> GETGQVIKSAVRSTVENTVQSTHSITTEATPALQAAETGATSNASDESMIETRNVVNTHGVAETSLEAFYGRAGLVAMFSTDGGIYRWYINFGEYVQLRAKLELLTYARFDMEFTIVAQVVNAQSKVQDFNVDYQVMFVPPGASVPENQDSYQWQSSCNPSVISNTGLPPARVSVPFMSSANAYSFSYDGYTQFGDTSGSSYGIVPSNYLGMLVVRTCEDLDGTRLRVRVYAKPKHVKGWIPRSPRMTPYKSRYTGVYTDTTKFCANRARITTAG;> SAEACGYSDRVAQLTLGNSTITTQEAANIVVGYGRWPTSLRDTDATAVDKPTQPGVSAERFYTLPSVQWTNSFKGHYWKLPDALSELGLFGQNLQFHYLYRGGWVIHVQCNATKFHQGTLLVVATPEHKIQSAESPAFARTNPGEQGAAYQFPFTFEDGTALGNALIYPHQWVNLRTNNSATLVLPYVNALPMDSGIRHNNWTLSVIPIVPLEYAAGATTYVPITVTIAPMCTEYNGLRAAVTQ;> GIPTLYTPGSGQFLTTDDFQTPCMLPKFQPTPVIDIPGEVKNFLEVVQVESLVEINNVESAEGVARYRIPLNVQDAMDGQIMALRVDPGIDGPMQSTLLGVFTRYYAQWSGSLDFTFMFCGTFMTTGKVIIAYTPPGGDQPTNRRQAMLGTHVVWDFGLQSSITLVVPWISSGHFRGTTLENTIYKYRYYEAGYITMWYQTNMVVPPNFPTTASILMFVAAQPNFSLRILKDRPDISQEGALQ;> MGAQMSKNTAGSHTTGTYATGGSNIHYTNINYYENAASNSLNKQDFTQDPEKFTRPVVDVMKEAAVPLKSP

Enteroviruses are responsible for a range of animal and human diseases. These non-enveloped viruses are constructed of an icosahedral protein capsid composed of 60 copies each of viral proteins VP1–4. VP1–3 are similar to each other (comprising a β-barrel with extended surface loops and termini) and form the capsid surface. Here we study EV-F3, a relatively benign bovine enterovirus which is our model system of choice. We firstly show that EV-F3 is dependent on GSH and that GSH stabilises the capsid.

In un-soaked EV-F3 virions, the I site is partially occupied by a ligand similar to GSH and to clarify the nature of the binding we performed two further structure determinations, firstly with CG (the GSH breakdown product) and secondly a competition soak with equal concentrations of both GSH and CG. We then determine high-resolution structures of complexes of GSH and its initial breakdown product Cys-Gly (CG) bound to EV-F3 and by a competition binding study demonstrate that GSH binds more strongly. The CG portion of GSH anchors the two adjacent protomers via not only these salt bridges, but also by additional H-bonding interactions with Y231 of protomer A and the carbonyl oxygen of W154 of protomer B via a bridging water molecule. Although the carboxylate group of the E residue of GSH makes no direct contacts with the I site, other portions of the residue contact D150 (protomer B) and, indirectly, R227 (protomer A) at the inter-protomer interface. Given that for GSH the strongest interactions are formed by the C-terminus of the ECG tripeptide, the binding of CG is not unexpected, the preference for GSH, however, confirms that additional binding energy is contributed by residue E, although its side chain can assume multiple conformations. We find that the binding site of both compounds is identical to that for a similar molecule that remains naturally attached to the virus, and to the binding site observed for the benzene-sulfonamide derivative in complex with Coxsackievirus B38, identifying the biological role for this binding site.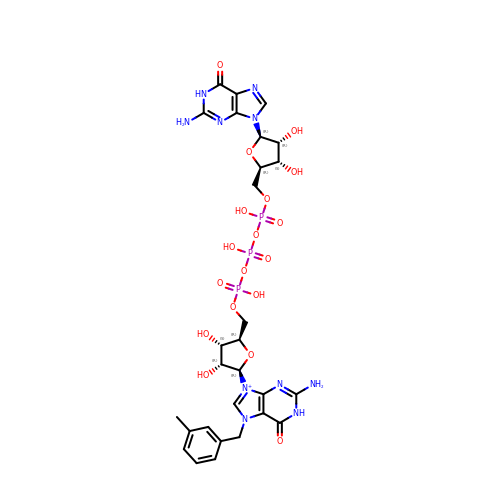[[(2~{R},3~{S},4~{R},5~{R})-5-[2-azanyl-7-[(3-methylphenyl)methyl]-6-oxidanylidene-1~{H}-purin-9-yl]-3,4-bis(oxidanyl)oxolan-2-yl]methoxy-oxidanyl-phosphoryl] [[(2~{R},3~{S},4~{R},5~{R})-5-(2-azanyl-6-oxidanylidene-1~{H}-purin-9-yl)-3,4-bis(oxidanyl)oxolan-2-yl]methoxy-oxidanyl-phosphoryl] hydrogen phosphate | C28 H36 N10 O18 P3 | PSRZFZZOIWOJQD-RTZOWOBBSA-O> MDFECQFVCELKELAPVPALLIRTQTTMSELGSLFEAGYHD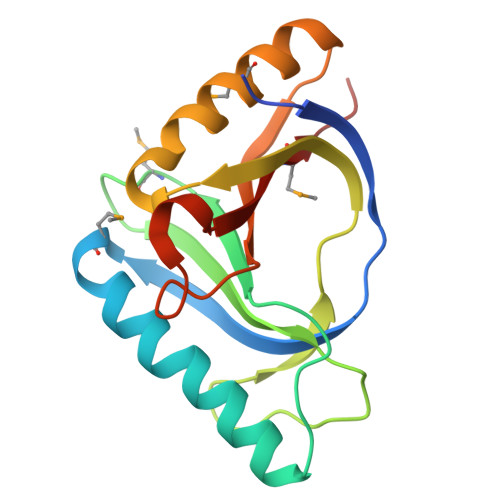ILQLLAGQGKSPSGPPFARYFGMSAGTFEVEFGFPVEGGVEGSGRVVTGLTPSGKAASSLYIGPYGEIEAVYDALMKWVDDNGFDLSGEAYEIYLDNPAETAPDQLRTRVSLMLHES> SSPSTTPINFHIN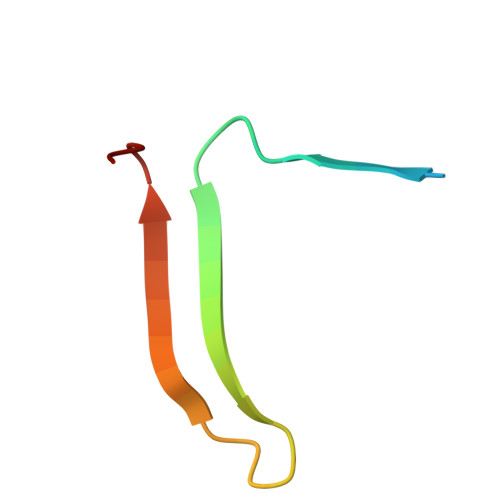KPFVFAIREKSTGVILFIGEIGEVKE>MQTAYVKYVDDTTGETLRQDDLHGYTDETIPYSTAEGIKKYEGDGYVLVSDGFKPGTKFGVGTPTYEVHFKHGMTHTDATDKNAEQKTVTETIHYVDENNQTVQPDSTTAVTFKRGYTTDNVTGKVVSYDPWTVDGNQADSKTFAAVPSPAVEGYTPNHQQINEFTVTPDSKDIVKT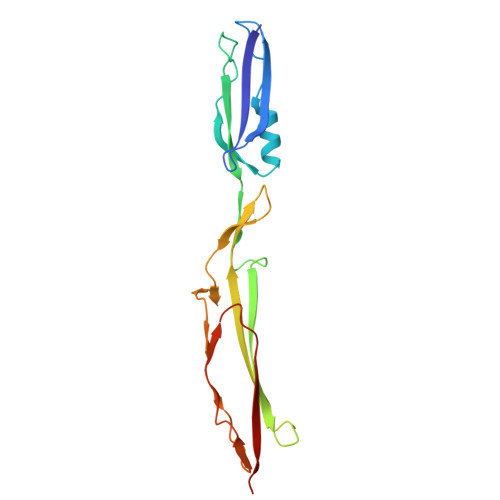VVYVGDP[2x]>MARKFFVGGNFKMNGSLESMKTIIEGLNTTKLNVGDVETVIFPQNMYLITTRQQVKKDIGVGAQNVFDKKNGAYTGENSAQSLIDAGITYTLTGHSERRTIFKESDEFVADKTKFALEQGLTVVACIGETLAEREANTINVVVRQLNAIADKVQNWSKIVIAYEPVWAIGTGKTATPEQAQEVHAE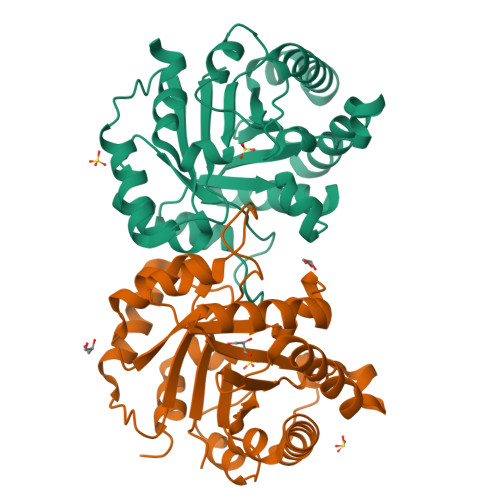IRKWATNKLGASVAEGLRVIYGGSVNGGNAKEFLKFHDIDGFLVGGASLKPEFHNIVNVHSL[4x]>EDSELISENMHMKLYMEGTVNDHHFKCTSEGEGKPYEGTQTMKIKVVEGGPLPFAFDILATSFMYGSKTFINHTQGIPDFFKQSFPEGFTWERITTYEDGGVLTATQDTSLQNGCLIYNVKINGVNFPSNGPVMQKKTLGWEASTEMLYPADSGLRGHSQMALKLVGGGYLHCSLKTTYRSKKPAKNLKMPGFYFVDRKLERI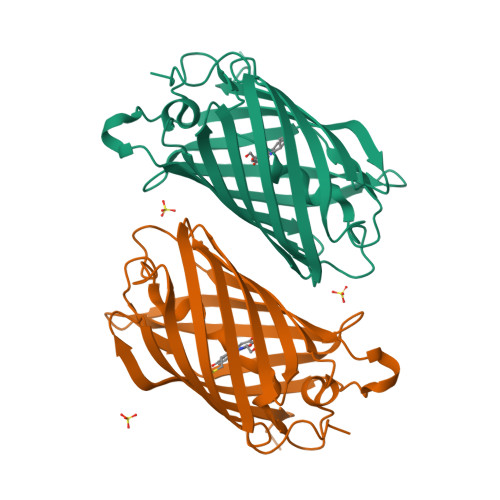KEADKETYVEQHEMAVARYCDLP[2x]>[2x]CGCAAA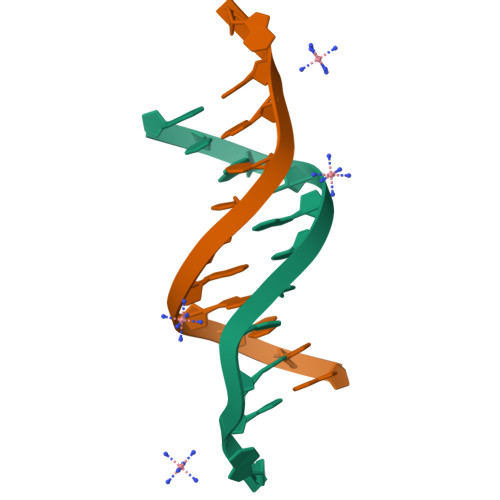TTXGCG>[3x]GSHMGLTFNSNNICIDDNINTLWTGVNPTTANCQIMASSESNDCK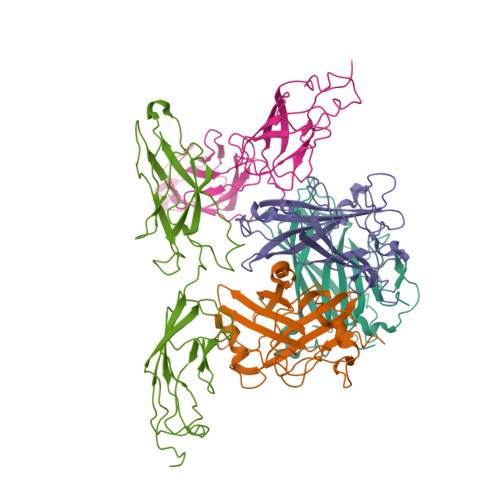LILTLVKTGALVTAFVYVIGVSNDFNMLTTHKNINFTAELFFDSTGNLLTSLSSLKTPLNHKSGQNMATGALTNAKGFMPSTTAYPFNVNSREKENYIYGTCYYTASDHTAFPIDISVMLNQRALNNETSYCIRVTWSWNTGVAPEVQTSATTLVTSPFTFYYIREDD;>[2x]QGAMEVLDINDNEPVFTQDVFVGSVEELSAAHTLVMKINATDADEPNTLNSKISYRIVSLEPAYPPVFYLNKDTGEIYTTSVTLDREEHSSYTLTVEARDGNGEVTDKPVKQAQVQIRILDVNDNIPVVENKVLEGMVEENQVNVEVTRIKVFDADEIGSDNWLANFTFASGNEGGYFHIETDAQTNEGIVTLIKEVDYEEMKNLDFSVIVANKAAFHKSIRSKYKPTPIPIKVKVKNVKEGI> MKQRIALSLLALGPLLLVPRVYAAADEPMANIVEKAVQPLLEEYRIPGMAVAVL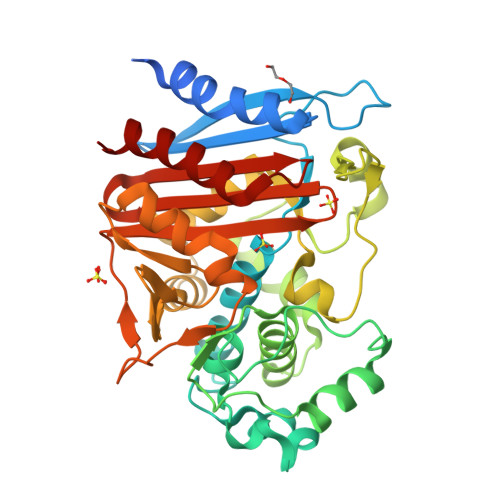KEGKPHYFNYGVANRESGRRISERTLFEIGSVSKTFTATLGTYAVVKGGFRLDDKVSQHAPWLQNSAFDRVTMAQLATYSAGGLPLQFPDAVDSNERMRQYYRQWSPLYAAGTHREYSNPSIGLFGHLAASTLGQPFRQLMSQTLLPKLDLQHTYLEVPDAAMVDYAYGYSKEDKPVRVNPGVLADEAYGIKTSAADLIKFVGANMTGSGDKAVQQALAMTRTGFYSVGEMTQGLGWESYAYPVTEQALLAGNSPAVSFKANPVKPFVAPRVMGNERLYNKTGSTNGFGAYVVFVPARGVGIVMLANRNYPIEARVKAAYAIMRHLAP> MWSHPQFEKMSSLPGSREPLLRVAVTGGTHGNEMCGVYLARYWLQNPGELQRPSFSAMPVLANPAATAACCRYLDRDLNRSCTLTFLGSTATPDDPYEVKRARELNQ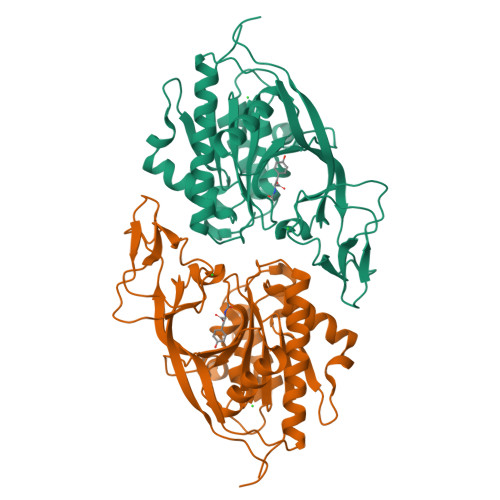LLGPKGTGQAFDFTLDLHNTTANTGVCLISESNISFNLHLCHYLQRQNPGMPCRLFLYEPAGTETFSVESISKNGICLAMGPQPQGVLRADLFSRMRALVASILDFIELFNQGMDLPAFEMDIYRNLGSVDFPRTADGDLAGTVHPQLQDHDFEPLRPGEPIFKLFSGEDVLYEGDSIVYPVFINEAAYYEKHVAFLKSEKIRVTVPALLRLTPRSTQTP>KEVCYGQLGCFSDEKPWAGTLQRPVKLLPWSPEDIDTRFLLYTNENPNNFQLITGTEPDTIEASNFQLDRKTRFIIHGFLDKAEDSWPSDMCKKMFEVEKVNCICVDWRHGSRAMYTQAVQNIRVVGAETAFLIQALSTQLGYSLEDVHVIGHSLGAHTAAEAGRRLGGRVGRITGLDPAGPCFQDEPEEVRLDPSDAVFVDVIHTDSSPIVPSLGFGMSQKVGHLDFFPNGGKEMPGCKKNVLSTITDIDGIWEGIGGFVSCNHLRSFEYYSSSVLNPDGFL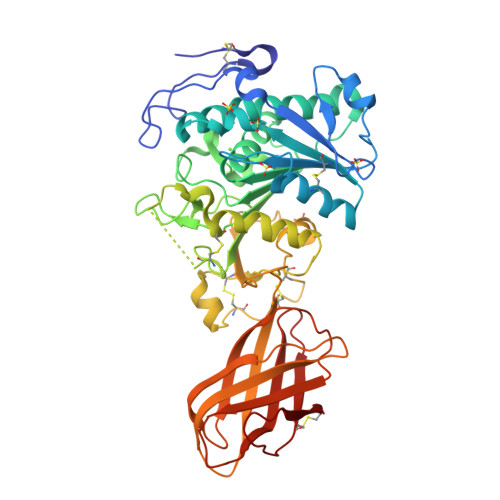GYPCASYDEFQESKCFPCPAEGCPKMGHYADQFKGKTSAVEQTFFLNTGESGQFTSWRYKVSVTLSGKEKVNGYIRIALYGSNENSKQYEIFKGSLKPDASHTCAIDVDFNVGKIQKVKFLWNKRGINLSEPKLGASQITVQSGEDGTEYNFCSSDTVEENVLQSLYPC[2x]> VKWSEDLANLPSIDTQHKRLVDYINDLYRAARRRDMDKAREVFDALKNYAVEHFGYEERLFADYAYPEATRHKEIHRRFVETVLKWEKQLA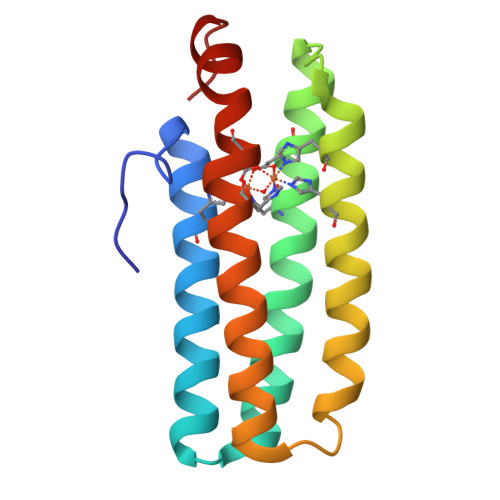AGDPEVVMTTLRGLVDWLVNHIMKEDKKYEAYLRERGVS> DYKDDDDAMANSASPEQNQNHCSAINNSIPLMQGNLPTLTLSGKIRVTVTFFLFLLSATFNASFLLKLQKWTQKKEKGKKLSRMKLLLKHLTLANLLETLIVMPLDGMWNITVQWYAGELLCKVLSYLKLFSMYAKAFMMVVISLDRSLAITRPLALKSNSKVGQSMVGLAWILSSVFAGPQLYIFRMIHLADSSGQTKVFSQCVTHCSFSQWWHQAFYNFFTFSCLFIIPLFIMLICNAKIIFTLTRVLGIDCSFWNESYLTGSRDERKKSLLSKFGMDEGVTFMFIGRFDRGQKGVDVLLKAIEILSSKKEFQEMRFIIIGKGDPELEGWARSLEEKHGNVKVITEMLSREFVRELYGSVDFVIIPSYFEPFGLVALEAMCLGAIPIASAVGGLRDIITNETGILVKAGDPGELANAILKALELSRSDLSKFRENCKKRAMSFSNIPRARLK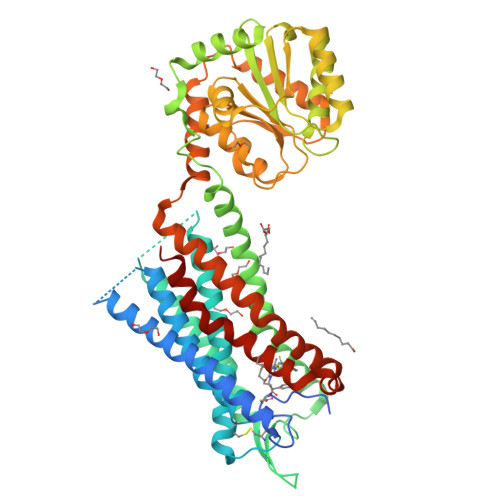TLKMTVAFATSFTVCWTPYYVLGIWYWFDPEMLNRLSDPVNHFFFLFAFLNPCFDPLIYGYFSLHHHHHHHHHH> MKLSPKAATLAERSAGLAFSLYQAMAKDQAVENILLSPVVVASSLGLVSLGGKATTASQAKAVLSAEQLRDEEVHAGLGELLRSLSNSTARNVTWKLGSRLYGPSSVSFAEDFVRSSKQHYNCEHSKINFRDKRSALQSINEWAAQTTDGKLPEVTKDVERTDGALLVNAMFFKPHWDEKFHHKMVDNRGFMVTRSYTVGVTMMHRTGLYNYYDDEKEKLQIVEMPLAHKLSSLIILMPNNVEPLERLEKLLTKEQLKIWMGKMQKKAVAISLPKGVVEVTHDLQKH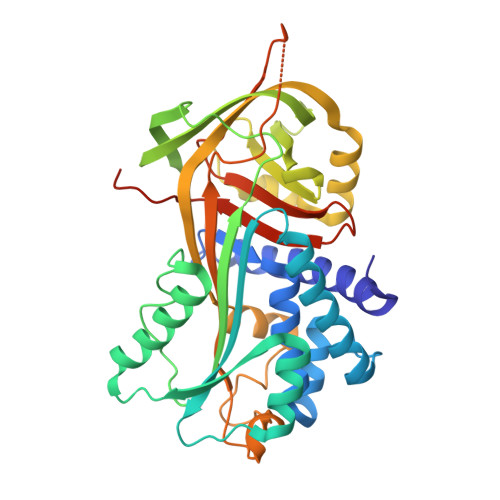LAGLGLTEAIDKNKADLSRMSGKKDLYLASVFHATAFEWDTEGNPFDQDIYGREELRSPKLFYADHPFIFLVRDTQSGSLLFIGRLVRPKGDKMRDELLEHHHHHH>[4x]GSEFGRKKIQIQRIT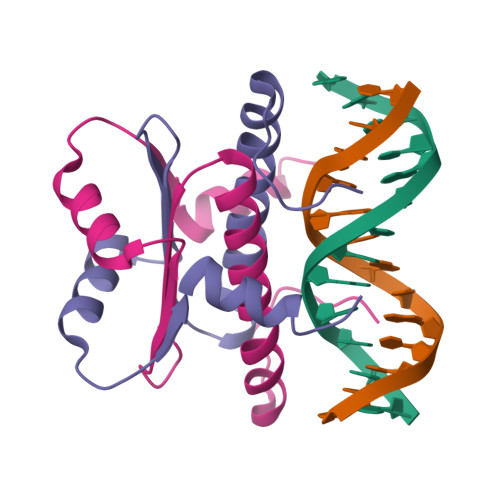DERNRQVTFTKRKFGLMKKAYELSVLCDCEIALIIFNHSNKLFQYASTDMDKVLLKYTEYNEPHESRTNADIIETLRKKGFNG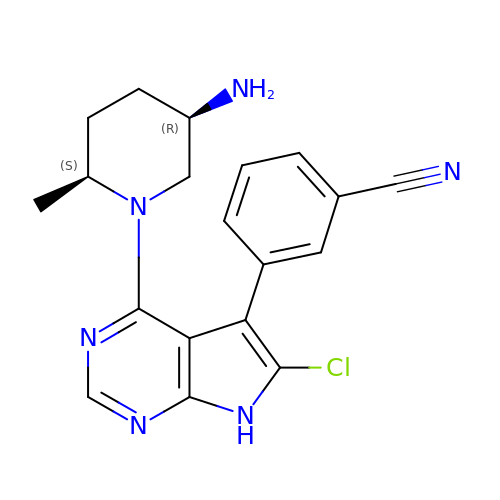(3P)-3-{4-[(2S,5R)-5-amino-2-methylpiperidin-1-yl]-6-chloro-7H-pyrrolo[2,3-d]pyrimidin-5-yl}benzonitrile | C19 H19 Cl N6 | IWFMUUASEIUTAN-SMDDNHRTSA-N>[2x]MLQPECSRSEEDLSDEKERKWEQLSRHWHTVVLASSDRSLIEEEGPFRNFIQNITVESGNLNGFFLTRKNGQCIPLYLTAFKTEEARQFKLNYYGTN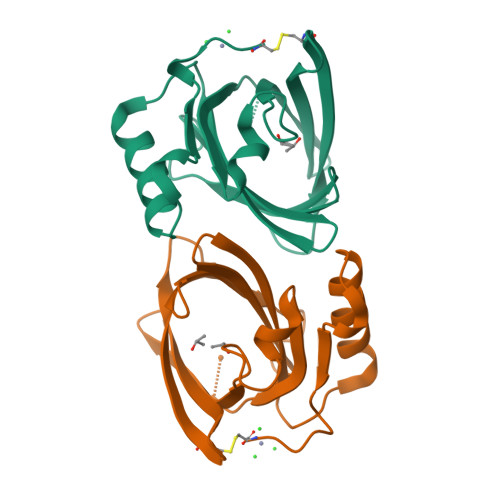DVYYESSKPNEYAKFIFYNYHDGKVNVVANLFGRTPNLSNEIKKRFEEDFMNRGFRRENILDISEVDHC>TNATGERNLALIQEVLEVFPETARKERRKHMMVSDPKMKSVGKCIISNRKSQPGVMTVRGCAYAGSKGVVFGPIKDMAHISHGPVGCGQYSRAGRRNYYTGVSGVDSFGTLNFTSDFQERDIVFGGDKKLSKLIEEMELLFPLTKGITIQSECPVGLIGDDISAVANASSKALDKPVIPVRCEGFRGVSQSLGHHIANDVVRDWILNNREGQPFETTPYDVAIIGDYNIGGDAWASRILLEEMGLRVVAQWSGDGTLVEMENTPFVKLNLVHCYRSMNYIARHMEEKHQIPWMEYNFFGPTKIAESLRKIADQFDDTIRANAEAVIARYEGQMAAIIAKYRPRLEGRKVLLYMGGLRPRHVIGAYEDLGMEIIAAGYEFAHNDDYDRTLPDLKEGTLLFDDASSYELEAFVKALKPDLIGSGIKEKYIFQKMGVPFRQMHSWDYSGPYHGYDGFAIFARDMDMTLNNPAWNELTAPWL[2x];>SQTIDKINSCYPLFEQDEYQELFRNKRQLEEAHDAQRVQEVFAWTTTAEYEALNFRREALTVDPAKACQPLGAVLCSLGFANTLPYVHGSQGCVAYFRTYFNRHFKEPIACVSDSMTEDAAVFGGNNNMNLGLQNASALYKPEIIAVSTTCMAEVIGDDLQAFIANAKKDGFVDSSIAVPHAHTPSFIGSHVTGWDNMFEGFAKTFTADYQGQPGKLPKLNLVTGFETYLGNFRVLKRMMEQMAVPCSLLSDPSEVLDTPADGHYRMYSGGTTQQEMKEAPDAIDTLLLQPWQLLKSKKVVQEMWNQPATEVAIPLGLAATDELLMTVSQLSGKPIADALTLERGRLVDMMLDSHTWLHGKKFGLYGDPDFVMGLTRFLLELGCEPTVILSHNANKRWQKAMNKMLDASPYGRDSEVFINCDLW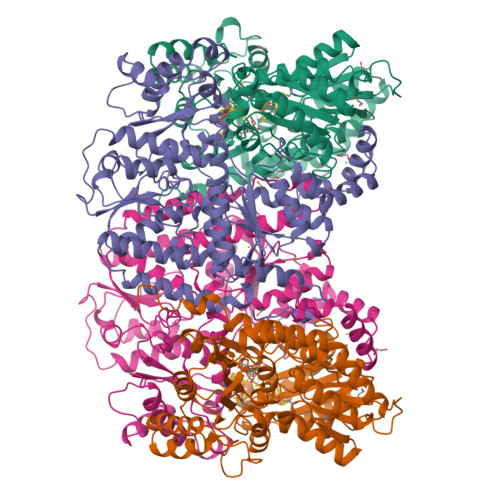HFRSLMFTRQPDFMIGNSYGKFIQRDTLAKGKAFEVPLIRLGFPLFDRHHLHRQTTWGYEGAMNIVTTLVNAVLEKLDSDTSQLGKTDYSFDLVR[2x]> MNIE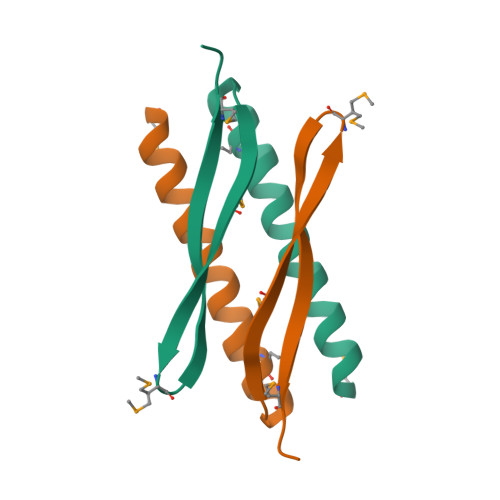ELKKQAETEIADFIAQKIAEMNKNTGKEVSEMRFTAREKMTGLESYDVKIKIMLEH>[2x]MGNYDSTPIAKSDRIKRLVDHLYAKMPEIEAARAELITESFKATEGQPVVMRKARAFEHILKNLPIIIRPEELIVGSTTIAPRGCQTYPEFSYEWLEAEFETVETRSADPFYISEETKKRLLAADAYWKGKTTSELATSYMAPETLRAMKHNFFTPGNYFYNGVGHVTVQYET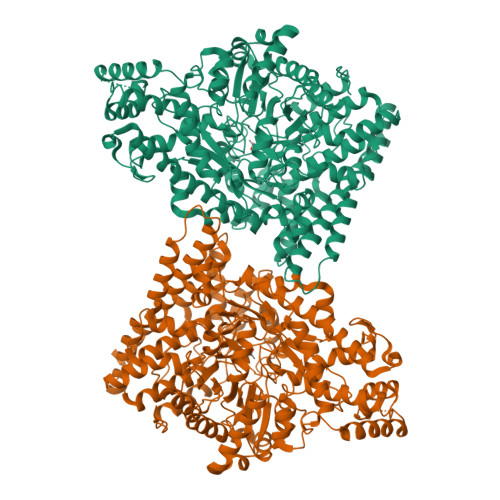VLAIGLNGVKEKVRKEMENCHFGDADYSTKMCFLESILISCDAVITYANRYAKMAEEMAEKETDAARRQELLTIARVCKNVPEFPAESFQEACQSFWFIQQVLQIESSGHSISPGRFDQYMYPYYEKDLKEGSLTREYAQELIDCIWVKLNDLNKCRDAASAEGFAGYSLFQNLIVGGQTVQGRDATNDLSFMCITASEHVFLPMPSLSIRVWHGSSKALLMRAAELTRTGIGLPAYYNDEVIIPALVHRGATMDEARNYNIIGCVEPQVPGKTDGWHDAAFFNMCRPLEMVFSNGYDNGEIASIQTGNVESFQSFDEFMEAYRKQMLYNIELMVNADNAIDYAHAKLAPLPFESCLVDDCIKRGMSAQEGGAIYNFTGPQGFGIANVADSLYTIKKLVFEEKRITMGELKKALEMNYGKGLDATTAGDIAMQVAKGLKDAGQEVGPDVIANTIRQVLEMELPEDVRKRYEEIHEMILELPKYGNDIDEVDELAREAAYFYTRPLETFKNPRGGMYQAGLYPVSANVPLGAQTGATPDGRLAHTPVADGVGPTSGFDISGPTASCNSVAKLDHAIASNGTLFNMKMHPTAMAGEKGLESFISLIRGYFDQQGMHMQFNVVDRATLLDAQAHPEKYSGLIVRVAGYSALFTTLSKSLQDDIIKRTEQADNR> AKLETVTLGNIGKDGKQT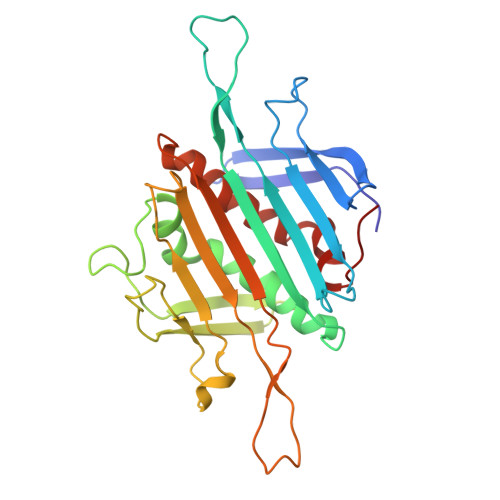LVLNPRGVNPTNGVASLSQAGAVPALEKRVTVSVSQPSRNRKNYKVQVKIQNPTACTANGSCDPSVTRQAYADVTFSFTQYSTDEERAFVRTELAALLASPLLIDAIDQLNPAYAYGGAKLETVTLGNIGKDGKQTLVLNPRGVNPTNGVASLSQAGAVPALEKRVTVSVSQPSRNRKNYKVQVKIQNPTACTANGSCDPSVTRQAYADVTFSFTQYSTDEERAFVRTELAALLASPLLIDAIDQLNPAY> GPKAEEEMSNELQNLDVQGKSKATGTGLVYVDAFTRFHCLWDASHPECPARVSTVMEMLETEGLLGRCVQVEARAVTEDELLLVHTKEYVELMKSTQNMTEEELKTLAEKYDSVYLHPGFFSSACLSVGSVLQLVDKVMTSQLRNGFSINRPPGHHAQADKMNGFCMFNNLAIAARYAQKRHRVQRVLIVDWDVHHGQGIQYIFEEDPSVLYFSVHRYEDGSFWPHLKESDSSSVGSGAGQGYNINLPWNKVGMESGDYITAFQQLLLPVAYEFQPQLVLVAAGFDAVIGDPKGGMQVSPECFSILTHMLKGVAQGRLVLALEGGYNLQSTAEGVCASMRSLLGDPCPHLPSSGAPCESALKSISKTISDLYPFWKSLQTFEGGPLSEVSPLPAPVCAEVKVSSPITGLVYDQRMMLHHNMWDSHHPELPQRISR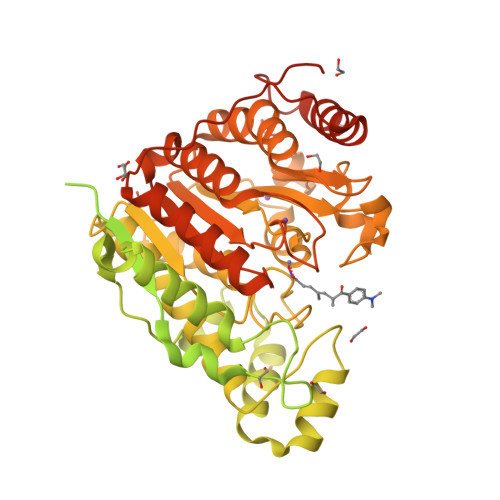IFSRHEELRLLSRCHRIPARLATEEELALCHSSKHISIIKSSEHMKPRDLNRLGDEYNSIFISNESYTCALLAAGSCFNSAQAILTGQVRNAVAIVRPPGHHAEKDTACGFCFFNTAALTARYAQSITRESLRVLIVDWDVHHGNGTQHIFEEDDSVLYISLHRYEDGAFFPNSEDANYDKVGLGKGRGYNVNIPWNGGKMGDPEYMAAFHHLVMPIAREFAPELVLVSAGFDAARGDPLGGFQVTPEGYAHLTHQLMSLAAGRVLIILEGGYNLTSISESMSMCTSMLLGDSPPSLDHLTPLKTSATVSINNVLRAHAPFWSSLRVNIPESLRLSLPSPKPKGKCTPGGKGKKSPRQS> MKFLFYLSADNLEIARKEVLVLAERYGWVEDYQFEERLLLLDYAGEKFFERLAYTNEVTKIYDICSVSELEQVFSEIPVYDRLCCVRVKGGKGKTALERKLGALLWKRGAKVSVSNPEIVYKVYIQDDKCYVGLLEFERDTRQFFLRRPDRRPFLMPSAIKPKLARALVNLTGVLEGETLLDPMCGTGSFLIEAGLMGINPIGIDFIEKIVRGCRVNLEYYGIEGSVLLGDAKNLPLRDESVRGIATDYPYLRSTKAAGTLDELYSKTSEEFERVLKKGGRAAIVTNIDVESFFSNFEIEMKTEER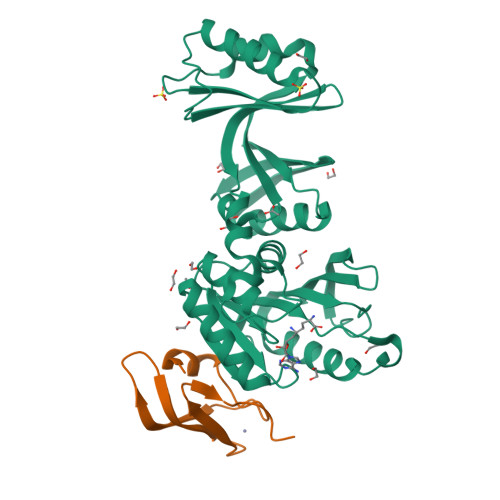VHGSLTRRIYLLRRHHHHHH;> MKRKLLEILACPLCKSELEVEVVEENEEEIISGKLVCSSCRAEFPIEDGIPDLRPPELRQ>MAMSPPTQDLHIPGRLDGKVALVTGSGRGIGAAVAVHLGLLGAKVVVNYANSPTHAQKVVDEIKQLGSDAIAIKADVRQVPEIVRLFDEAVAHFGQLDIAVSNSGVVSFGHLKDVTEEEFDRVFSLNTRGQFFVAREAYKHLNNGGRIIMTSSNTSRDFSVPKFSLYSGSKGAIDSFVRIFSKDCGDKKITVNAVAPGGTVTDMFHDVSQHYIPNGETYTPEERQKMAAHASPLHRNGFPEDIARVVGFLVSAEGEWINGKVLTVDGGAAALEHHHHHH[4x]

In this study, an anthrol reductase (CbAR) from Cercospora sp. JNU001 with the ability for asymmetric reduction of various bulky substrates was identified and characterized. It belongs to the SDR superfamily and shares the highest sequence identity of 86.6% with 17β-HSDcl from Curvularia lunata. Similar to other SDRs, the overall structure of CbAR monomer contains nine α-helices and two sets of β-sheets (β1-β7), in which continuous β-sheets and seven α-helices constitute the standard Rossmann-fold motif responsible for NADPH binding and the C-terminal domain constitutes a substrate binding pocket. In both of crystal structures of CbAR-NADP+ and CbAR-NADP+-Emodin, the catalytic triad (Ser151, Tyr165 and Lys169) is well observed.

Indeed, CbAR-H162F, CbAR-Y210F and CbAR-Y210A variants could enhance the catalytic activity towards 1e, with 44.7, 4.6 and 3.2-fold increase, respectively. To reveal the exclusive stereoselectivity for 2,2-disubstituted 1,3-cyclodiketones by CbAR-H162F, crystal structure of CbAR-H162F-NADP+-1e complex was successfully obtained and refined to 2.75Å resolution. Its overall structure is very similar with CbAR-emodin complex. The “gate” region (from residue 209 to 216) is visible, but the conformation is different. Importantly, although the electron density map of 4-methylbenzyl group of 1e was unclear, probably due to the considerable mobility of the flexible benzyl groups, the 2-methyl-cyclopentane-1,3-dione part of 1e is clearly observed and well localized to the active site of CbAR-H162F. Notably, we observed that only two of the possible four binding sites in the crystallographic asymmetric unit are occupied by 1e. One carbonyl group of 1e forms the hydrogen-bond interaction with the amino group of Gly197. In addition, it shows that the 2-methyl group of 1e orients towards co-factor NADP+. In all, these observations well demonstrate the exclusive stereoselectivity for 2,2-disubstituted 1,3-cyclodiketones catalyzed by CbAR-H162F to deliver corresponding (2S, 3S)-ketols. All of them could be efficiently converted into the corresponding (2S, 3S)-ketols (2e–2i) with higher than 93% conversion and 99% ee by CbAR-H162F, whose conversions were better than that of wild-type CbAR.>MLVSVYLALLVACVGQAHSQANLMRLKSDLFNRSPMYPGPTKDDPLTVTLGFTLQDIVKVDSSTNEVDLVYYEQQRWKLNSLMWDPNEYGNITDFRTSAADIWTPDITAYSSTRPVQVLSPQIAVVTHDGSVMFIPAQRLSFMCDPTGVDSEEGVTCAVKFGSWVYSGFEIDLKTDTDQVDLSSYYA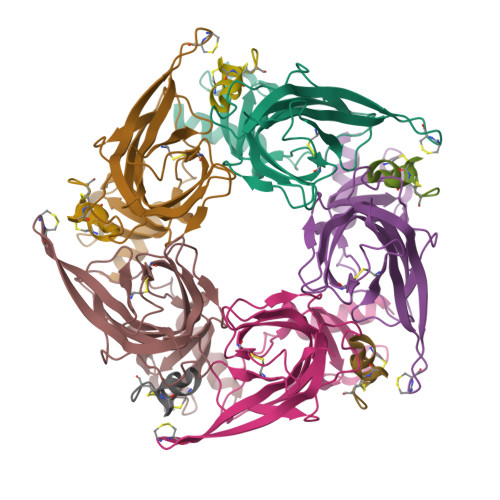SSKYEILSATQTRQVQHYSCCPEPYIDVNLVVKFRERRAGNGFFRNLFD[5x];>GCCSHPACAGNNQHICX[5x]> SAMGWSHPQFEKMAESASKAAPGERVVIGITFGNSNSSIAHTVDDKAEVIANEDGDRQIPTILSYVDGDEYYGQQAKNFLVRNPKNTVAYFRDILGQDFKSVDPTHNHASAHPQEAGDNVVFTIKDKAEEDAEPSTLTVSEIATRYLRRLVGAASEYLGK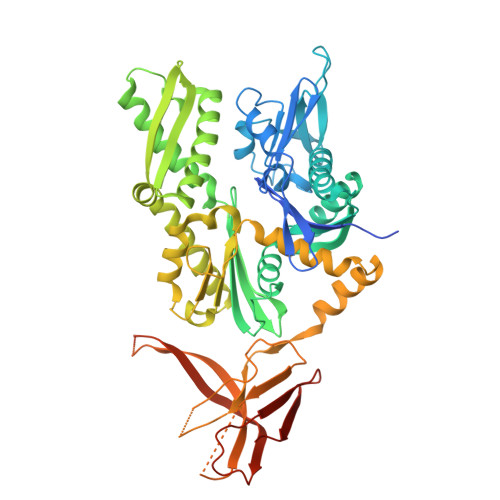KVTSAVITIPTNFTEKQKAALIAAAAAADLEVLQLISEPAAAVLAYDARPEATISDKIIVVADLGGSRSDVTVLASRSGMYTILATVHDYEYHGIALDKVLIDHFSKEFLKKNPGAKDPRENPRSLAKLRLEAESTKRALSRSTNASFSVESLIDGLDFASTINRLRYETIARTVFEGFNRLVESAVKKAGLDPLDVDEVIMSGGTSNTPRIAANFRYIFPESTRILAPSTDPSALNPSELQARGAALQASLIQEFETEDIEQSTHAAVTTMPHVTNAIGVVSVSESGEEKFVPIIAPETAVPARRTVHLDAPKEGGDVLVKVVEGSTHINVIKPEPKAKEDGETKEKTEDADDDGDFDDDDEEEEEEEEEEEKREKVWKIGSTLAEAAVRGVKKGAKVEVTINVNTDLTVIVTAREVGGKGGVRGTLSA Here we used a modified form of graphene, in conjunction with a stable grid made of gold, to control these surface effects. Functionalized graphene-on-gold grids improve the reliability of specimen preparation and enhance image quality. To address this problem we developed a method to produce multifunctional and ultrastable graphene supports with tunable surface properties for cryoEM. To demonstrate that these supports are suitable for high-resolution structure determination, we used an amylamine-functionalized graphene on gold support to determine the structure of horse spleen apoferritin.

The reconstruction reached 2.1-Å resolution (0.143 Fourier shell correlation [FSC]) from 41,202 particles with standard data collection and processing. The resolution of the reconstructed map, which is equivalent to the highest reported to date for this specimen, but required about half as many data, is demonstrated by clear densities for side chains in the map. This includes complete aspartate and glutamate residues, for which densities beyond the Cβ are often absent from EM maps. The decay rate of high-resolution information with fluence after the first 5–10 e−/Å2 of irradiation in this dataset is similar to measurements of radiation damage in 2D protein crystals. Adding a graphene layer to an all-gold support reduced particle movement by a factor of 2 during electron irradiation. Compared with graphene-on-carbon supports, graphene-on-gold supports reduced particle movement by a factor of 3. Importantly, besides reducing the rate of random (uncorrelated) particle motion, the addition of the graphene layer also reduces the movement during the first few electrons of irradiation, improving the quality (B-factor) of these initial frames, in which the molecules are less damaged by the beam. We posit that the twofold reduction in the initial movement of the particles in ice is due to the graphene layer restricting the bulk movement of the thin film of ice within each hole.

>[24x]SQIRQNYSTEVEAAVNRLVNLYLRASYTYLSLGFYFDRDDVALEGVCHFFRELAEEKREGAERLLKMQNQRGGRALFQDLQKPSQDEWGTTLDAMKAAIVLEKSLNQALLDLHALGSAQADPHLCDFLESHFLDEEVKLIKKMGDHLTNIQRLVGSQAGLGEYLFERLTLK> 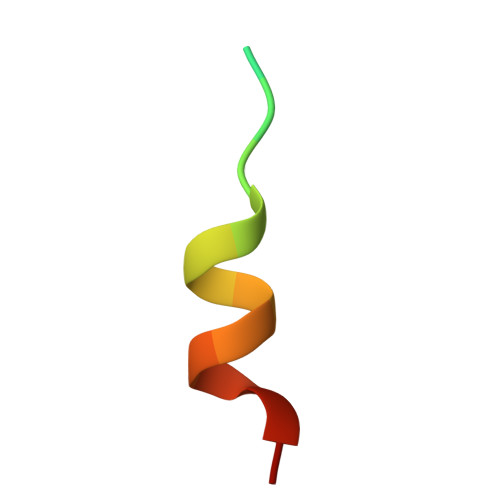GGGKEKHKILHRLLQDSS Rhodotorula dairenensis β-fructofuranosidase is a highly glycosylated enzyme with broad substrate specificity that catalyzes the synthesis of 6-kestose and a mixture of the three series of fructooligosaccharides (FOS), fructosylating a variety of carbohydrates and other molecules as alditols. RdINV subunit is composed of two domains, similar to the rest of the reported fungal β-fructofuranosidases within GH32. The β-propeller catalytic domain contains residues 185 to 487 and is constituted by five blades (I-V), each involving four antiparallel β-strands (ABCD) with a “W” topology. The β-sandwich domain, extending from residue 495 to 673, is composed of twelve β-sheets ordered in two six-stranded clusters of antiparallel β-strands.

A single homogeneous band with a molecular weight of 85–90 kDa was observed in the SDS gel after a combined α1-2,3,6 mannosidase/Endo H enzymatic treatment, which allowed crystal structure determination at 2.05 Å resolution. RdINV was indexed in the C2221 space group, with two molecules in the asymmetric unit and 37.4% solvent content. RdINV presents a homodimer arrangement that corresponds to the two molecules described within the crystallographic asymmetric unit. They are associated in a “butterfly” shape to form a tight homodimer related by a well-defined two-fold symmetry axis, similar to that previously described in the SoFfase homolog. The interface is mostly formed by blades IV and V from each catalytic domain and the β7β8 loop from their corresponding β-sandwich domain through twelve hydrogens bonds (monomer description is included in the following paragraph). Each polypeptide chain is composed of 675 residues, but the absolute lack of electron density prevented the model building of the sequence before Ser140. At least six O-glycosylation sites (Thr146, Ser147, Ser151, Ser153, Thr161, Thr163) located at the beginning of the chain and 13 N-glycosylation sites (Asn197, Asn240, Asn255, Asn263, Asn341, Asn350, Asn405, Asn475, Asn505, Asn514, Asn525, Asn535, Asn546) distributed over the two domains were clearly defined at the electron density map within each monomer. A PEG and a glycerol molecule were captured in the catalytic site of chain A at subsites −1 and +1, whereas glycerol and Bis-Tris were trapped in chain B. A remarkable feature is the presence of a di-sulfur bridge linking Cys143 to Cys555 that connects the prominent Pro551-Pro566 loop to the visible portion of the N-terminus and possibly helps in keeping the structural integrity of the Ser140-Asp168 region that has been observed in the crystal. Moreover, the Bis-Tris molecule shows one of its hydroxyl groups very close to the fructose and, thus, is in a proper position to act as an acceptor substrate in a putative transfructosylating reaction.

>MKFTLLSVVAIAAAASDSYAAPAASSLAGPVTTGVFSAVSAIPSFATNLSGQVASATSTVLSGSTASGSSATAAPSASASGASSMQSMASSLSGSAFSPSSMMPIASGNMTMPNMTSSASASSAASTATGVAGGAGSNSSSSCAPTSLPASATELPTTVPTGTVITGDYTGSYRPQVHYSPPKGFMNDPNGCHRDRNGTYHLYYQYNPLEYVAGNQHWGHATSDDLYHWTNQPIAIFPPNSTSQVFSGSAVLDPNNTSGFFPNTTDGVVAVYTLNTPTLQVQEVAYSTDGGYNFTPYENNPVLSVGSNQFRDPKVFWYEDHWVMAVAAANDFTIEIYTSPNLTSWTFASNFTHHGLLGLAYECPNLVQVPFQDDPSKSAWLMYISINPGAPLGGSVGQYFPGDFNGTHFVAYDSAARIADFAKDNYASQWFADTENGESISIAWASNWQYTQQVPTSAQAFRSAMSLPRRNYLTNITRLGWDLVSLPYDLSPVVGPSLLSSSEANSTADVDFTNVTSNAVWFSLNVTLPDAAIQNASLISADASINITFLPSTKCSSSSGSGSDSPAATLTYFYAGLTNGALALTRPAASSSWGAENPFFTDKFSYTLVDPLTSLVGVFDRSMLEVFVNEGAHSATMLVFPDSPVGSMKVATGGLPEGTQVNLQVNGLESTWQSS[2x]> VNECAEEGYCSQGCTNSEGAFQCWCEAGYELRPDRRSCKALGPEPVLLFANRIDIRQVLPHRSEYTLLLNNLENAIALDFHHRRELVFWSDVTLDRILRANLNGSNVEEVVSTGLESPGGLAVDWVHDKLYWTDSGTSRIEVANLDGAHRKVLLWQSLEKPRAIALHPMEGTIYWTDWGNTPRIEASSMDGSGRRIIADTHLFWPNG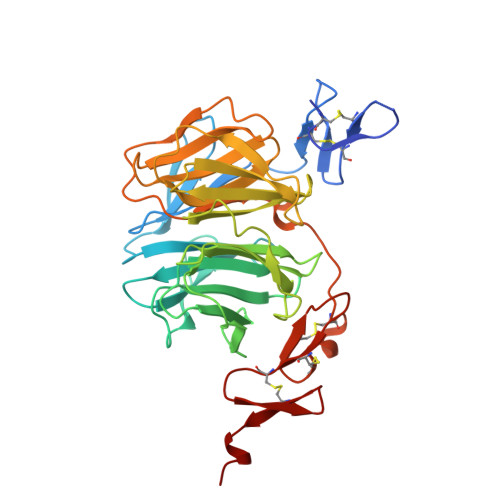LTIDYAGRRMYWVDAKHHVIERANLDGSHRKAVISQGLPHPFAITVFEDSLYWTDWHTKSINSANKFTGKNQEIIRNKLHFPMDIHTLHPQRQPAGKNRCGDNNGGCTHLCLPSGQNYTCACPTGFRKINSHACALEVLFQG> GCCCGGAUGAUCCUCAGUGGUCUGGGGUGCAGGCUUCAAACCUG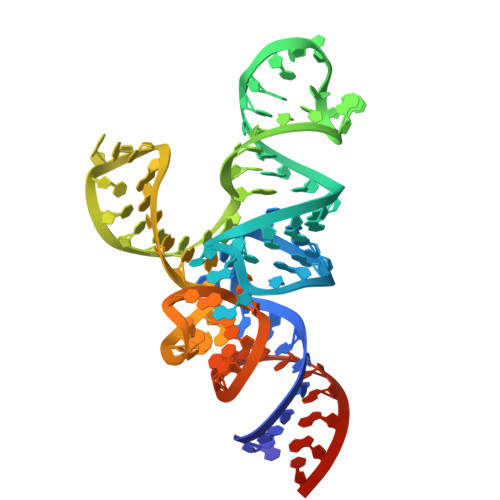UAGCUGUCUAGCGACAGAGUGGUUCAAUUCCACCUUUCGGGCGCCA>GPLGSPLTASMLASAPPQEQKQMLGERLFPLIQAMHPTLAGKITGMLLEIDNSELLHMLESPESLRSKVDEAVAVLQAHQAKEAAQKA[2x];>SNLNPNAKE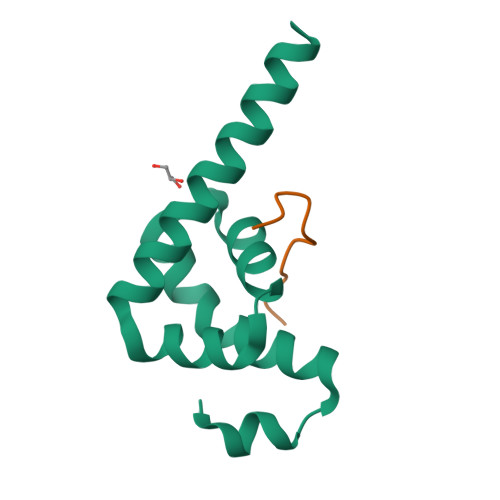FVPGVK[2x]>MTATEPTEKILPSPDYVQSLARGLAVIRCFDHRNQRRTLSDVARATDLTRATARRFLLTLVELGYVATDGSAFWLTPRVLELGYSYLSSLSLPEVAQPHLEKLSHKVHESSSVSILDGADIVYVARVPVSRIMTVGITIGTRLPAYATSMGRVLLAGLPDDELDAYLEKLDIQRLTERTITARDELKAAILAVRADGICVLDQELEAGLRSMAAPIRGASGLTVAAVNISTPAARYSLEDLHSDLIP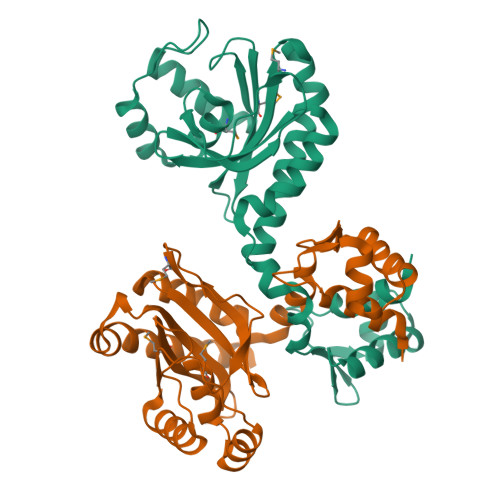SLRVTATDIEQDLATVNR[4x]>MAITKINDCFELLSMVTYADKLKSLIKKEFSISFEEFAVLTYISENKEKEYYFKDIINHLNYKQPQVVKAV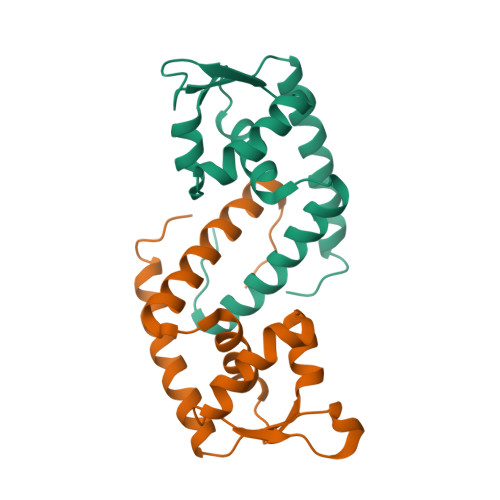KILSQEDYFDKKRNEHDERTVLILVNAQQRKKIESLLSRVNKRITEANNEIEL[2x]> GSGSTVANNVTNPNVDMTGWLLANSASAILDKSGISQQEVNDLTAHLDTYLKKMNILPSEDISTVLNQVKSDGVKKLHVKSREYIVNSLIEFTDDFEFVNETGTVFNFGDTGGFYASGSHTQITTLASDIVKNQSQSFDVADASQIQKGDWLVIYCTDDFSYSPYRNYYRKGEFVEVASVSGNTVKFFGRAYDNYLTSENIVILKVNPINFKFNYLKTVSTDNNPNVPLVIDYARNFETGYFENKGGKFAGLRLRRCFNFNIAINSAKNNAPANTLNYGIQISNCQNYNYFGGSNNSTRHAVAIGGDGDLGCVPCRNGYVSGAILHSETDTSGADMHGNVERTVYDHCTTNYATFGAGDNEYSNCDIYEREGQGCVLIAEPRGGEFKLTNNTYYTKTPLNSWSLVHGIIEKQLHEDLTVKLDGGCINGVGGASAGIVTIRQSNALNEALTKKVNVHITGGVSCDFDALRHWAWVEDGTIGRYTVPIGYIIVDDVVNTKDTANPYLIYPSQS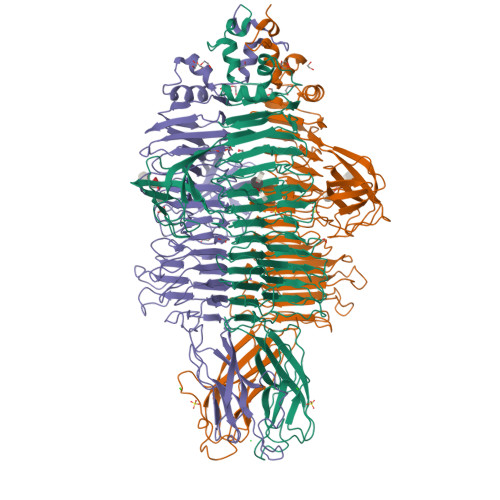TLATNVKTRQMLQQGVVSVTSAVNNTATRANVINLKYKYSKAPNVIVSVGNLVGSASWDATFFNEDTNVEPLRTPTPVNSLVAIDQVRPAILWNKKVVTPKTFNLYWESGIREI> MQHYLHIRPAPSDNLPLVDLIEHPDPIFDPKEKDLNETLLRSLLGGHYDPGFMATSPPEDRPGGGGGAAGGAEDLAELDQLLRQRPSGAMPSEIKGLEFSEGLAQGKKQRLSKKLRRKLQMWL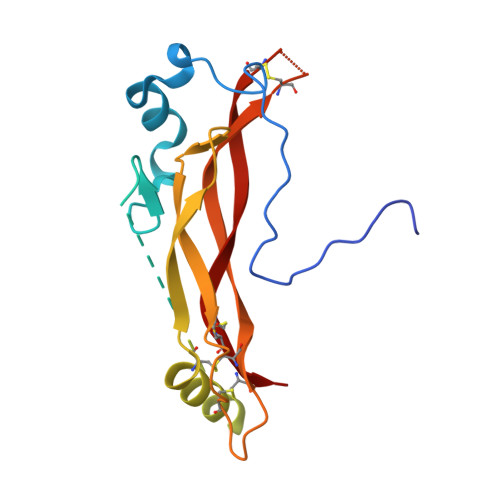WSQTFCPVLYAWNDLGSRFWPRYVKVGSCFSKRSCSVPEGMVCKPSKSVHLTVLRWRCQRRGGQRCGWIPIQYPIISECKCSC> MQFRLFSFALIILNCMDYSHCQGNRWRRS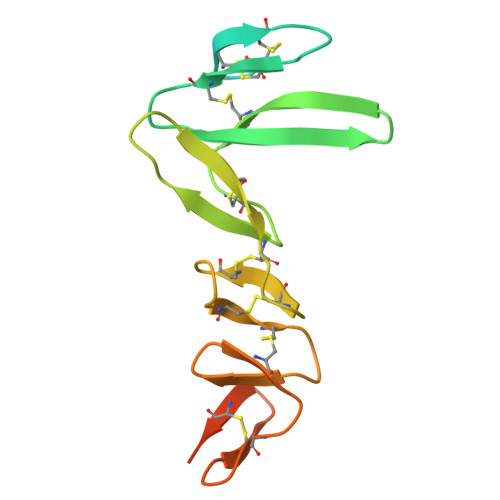KRASYVSNPICKGCLSCSKDNGCSRCQQKLFFFLRREGMRQYGECLHSCPSGYYGHRAPDMNRCARCRIENCDSCFSKDFCTKCKVGFYLHRGRCFDECPDGFAPLEETMECVEENLYFQGHHHHHHHHHH>[2x]MTDAATAPTSIDLRAEYEGSGAKEVLEELDRELIGLKPVKDRIRETAALLLVERARQKLGLAHETPTLHMSFTGNPGTGKTTVALKMAGLLHRL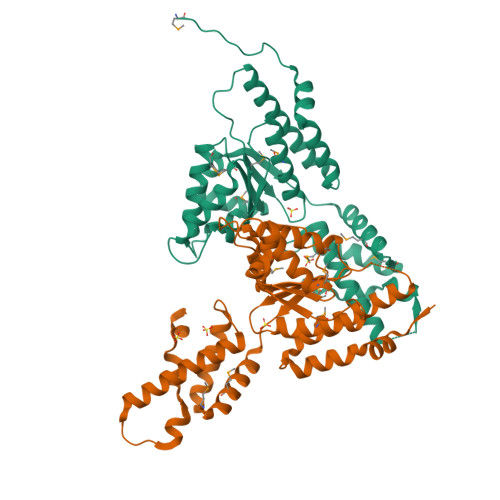GYVRKGHLVSVTRDDLVGQYIGHTAPKTKEVLKRAMGGVLFIDEAYYLYRPDNERDYGQEAIEILLQVMENNRDDLVVILAGYADRMENFFQSNPGFRSRIAHHIEFPDYSDEELFEIAGHMLDDQNYQMTPEAETALRAYIGLRRNQPHFANARSIRNALDRARLRQANRLFTASSGPLDARALSTIAEEDIRASRVFKGGLDSERRAAEALAR> SERFPNDVDPIETRDWLQAIESVIREEGVERAQYLIDQLLAEARKGGVNVAAGTGISNYINTIPVEEQPEYPGNLELERRIRSAIRWNAIMTVLRASKKDLELGGHMASFQSSATIYDVCFNHFFRARNEQDGGDLVYFQGHISPGVYARAFLEGRLTQEQLDNFRQEVHGNGLSSYPHPKLMPEFWQFPTVSMGLGPIGAIYQAKFLKYLEHRGLKDTSKQTVYAFLGDGEMDEPESKGAITIATREKLDNLVFVINCNL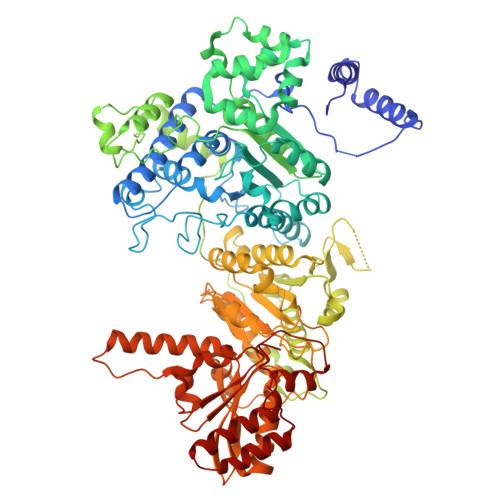QRLDGPVTGNGKIINELEGIFEGAGWNVIKVMWGSRWDELLRKDTSGKLIQLMNETVDGDYQTFKSKDGAYVREHFFGKYPETAALVADWTDEQIWALNRGGHDPKKIYAAFKKAQETKGKATVILAHTIKGYGMGDAAEGKNIAHQVKKMNMDGVRHIRDRFNVPVSDADIEKLPYITFPEGSEEHTYLHAQRQKLHGYLPSRQPNFTEKLELPSLQDFGALLEEQSKEISTTIAFVRALNVMLKNKSIKDRLVPIIADEARTFGMEGLFRQIGIYSPNGQQYTPQDREQVAYYKEDEKGQILQEGINELGAGCSWLAAATSYSTNNLPMIPFYIYYSMFGFQRIGDLCWAAGDQQARGFLIGGTSGRTTLNGEGLQHEDGHSHIQSLTIPNCISYDPAYAYEVAVIMHDGLERMYGEKQENVYYYITTLNENYHMPAMPEGAEEGIRKGIYKLETIEGSKGKVQLLGSGSILRHVREAAEILAKDYGVGSDVYSVTSFTELARDGQDCERWNMLHPLETPRVPYIAQVMNDAPAVASTDYMKLFAEQVRTYVPADDYRVLGTDGFGRSDSRENLRHHFEVDASYVVVAALGELAKRGEIDKKVVADAIAKFNIDADKVNPRLA(1S)-N-{(1S)-7,7-dihydroxy-1-[4-(2-methylquinolin-6-yl)-1H-imidazol-2-yl]nonyl}-6-methyl-6-azaspiro[2.5]octane-1-carboxamide 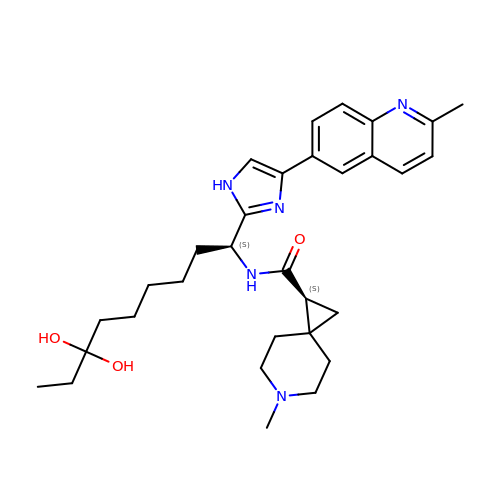| C31 H43 N5 O3 | TUQSZAQBKOXAIB-RSXGOPAZSA-N> RWAPIPCSMLENSLGPFPLFLQQVQSDTAQNYTIYYSIRGPGVDQEPRNLFYVERDTGNLYCTRPVDREQYESFEIIAFATTPDGYTPELPLPLIIKIEDINDNEPVFTQDVFVGSVEELSAAHTLVMKINATDADEPNTLNSKISYRIVSLEPAYPPVFYLNKDTGEIYTTSVTLDREEHSSYTLTVEARDGNGEVTDKPVKQAQVQIRILDVNDNIPVVENKVLEGMVEENQVNVEVTRIKVFDADEIGSDNWLANFTFASGNEGGYFHIETDAQTNEGIVTLIKEVDYEEMKNLDFSVIVANKAAFHKSIRSKYKPTPIPIKVKVKNVKEGIHFKSSVISIYVSESMDRSSKGQIIGNFQAFDEDTGLPAHARYVKLEDRDNWISVDSVTSEIKLAKLPDFESRYVQNGTYTVKIVAIS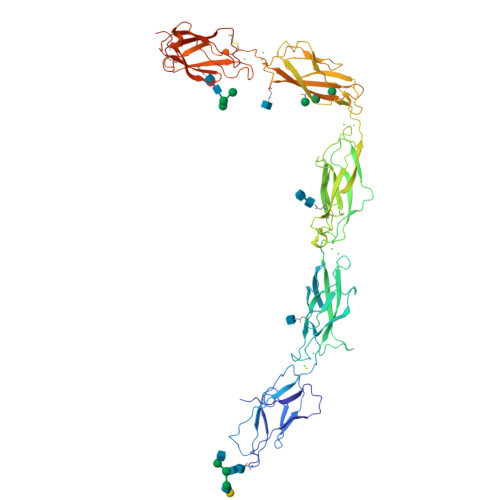EDYPRKTITGTVLINVEDINDNCPTLIEPVQTICHDAEYVNVTAEDLDGHPNSGPFSFSVIDKPPGMAEKWKIARQESTSVLLQQSEKKLGRSEIQFLISDNQGFSCPEKQVLTLTVCECLHGSGCREAHHHHHH(R)-N-(1-METHYL-HEXYL)-FORMAMIDE 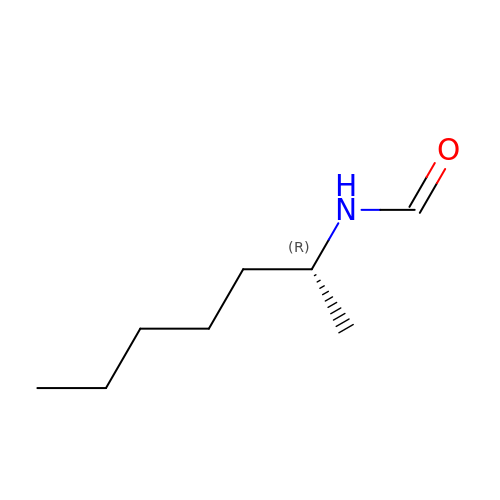| C8 H17 N O | GFVRKPKAQHTAQK-MRVPVSSYSA-N5-methyl-4H-1,2,4-triazole-3-thiol | C3 H5 N3 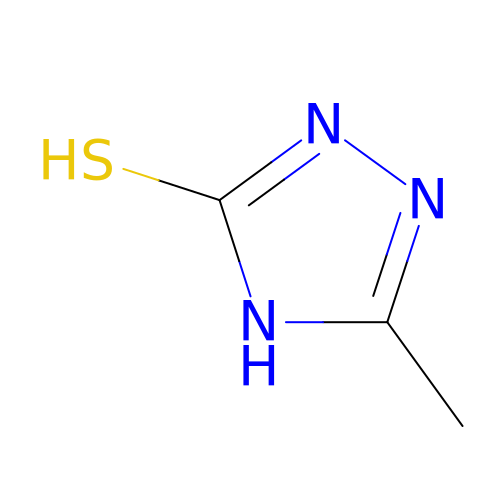S | OUZCWDMJTKYHCA-UHFFFAOYSA-N>MASSTAAPPAAVPAIETAAPPSPEPRDSVSVNEGGDASSAQAGAAVGSTIIVGAPELEKEYSDLNFAQVARDEGRRCLLMCVAFAIAIAHLYIYPALFGVRIVDQAEVPAEERTYFHHGWTAMLVIFFIEGVTVFLKVCSTRKTRWLEKAVLQKLDGNIGVLIGEYIVVAATYIIMGANLIPVFEEPRSGRRVYAVRYMEWTIDACGLVYLDCRILFGMPFSKFRMLLVYSVLYMLFGLWAALASTWMWYAIFLSASWFFFGLVCYYYWTFHRQNPSPLQQFGRAPIKQAILVFVIVWWVLYGVLFMLCFQAPDVVPQWLEQLLWTGMDVVMKLSHT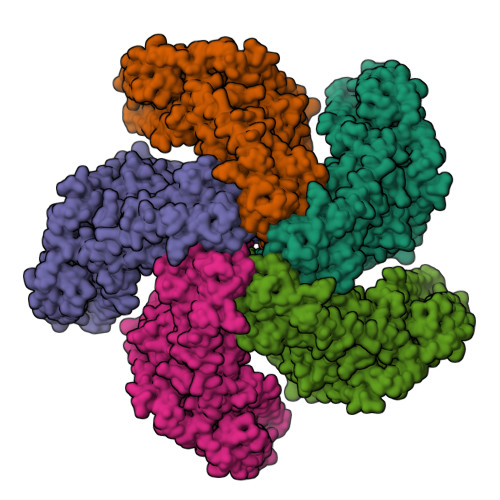VVLMAWRETQWEIDAVVDRQKVEAGRAIAQLDHQRAIHERDLVRLRSRVYYGEHIKSEEEIKSEEVISRSLRARKSRQGQDGTEPSSALSGASSTKEPPALEENSGSAAPSWTAVLAKGKATSSPFARVNKIFMREAGLCLVLCLAFVVALLHLPVYSEWFGVEVLDAEAVPHDELGFFHHGWTTMLVVFLIESITVLLKVWSTWHDPRLAENVAQQLSGNLGVLIAEYLVVGATYVILGYNLMPVFVVHRPGVASRRVYAVRYMEWAVDATGLIWLDCHCLFSRNFNEFRMAIVWTVAYMLFGLWSALASTWAWYWAFLLASWAAFLIVCLILVRFLRQDPYPHQPFGKTSVKPCILAFIIGWWVLYGILFMVCFQAPDAVPQWLEQFLWTGMDVVMKLSHTVVLMAWRTTEWNVCELHGRNQAEKSKKSLLNEGSHARQEKQQLEAIMLEGGGVEAAGRVGSVSFAPSSSRRRKESDSTNWTATPGLRVDLSSMVRLEGQLAQGLVTDVHRKGMMRSEDLAELKRLEESGFLQAQQHRNWESQTREMTFLAHGINHIAYDPRSWMKTLTAVRGRAPTSFLLWVVLIESSIVLALSKFFGESFDLGVSSGIHSLFGVLVSFLVVFRTQAAFKKWWSGRSAVSSLVQMSRTFAQQVCAYVKDEAYVNRMVRYSIATVVATRCHLRNTRIDPAMLLGVLKEEEIEELNRQKNLPFYTAWVIRSTLAEAVAEGACLPLHMAIENAIKAIEQSIADAERLLTPMPFTYVVHVRTFLFIYLMGLPFILVEDLGWLMLVAVSFLGYLMIGLENTAVQLENPFGTDCNHHPLDLYCLEVSQDLLHLLDLRASAKAQ[5x]> MFADRLFNAMERNEPAPGMVLVAAPSMESEDFARSVILIIEHSEYATFGVNLASRSDVAVFNVIPEWVPCVTKPQALYIGGPLNQQSVVGVGVTAQGVDAARVDNLTRLANRLVMVNLGADPEEIKPLVSGMRLFAGHAE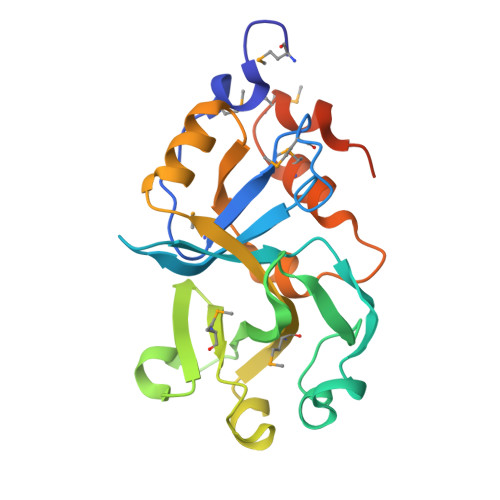WAPGQLAQEIENGDWFVAPALPSDVTAPGSVDVWGDVMRRQPMPLPLYSTFPVNVVGENLEHHHHHH>MKRRVVITGVGVRAPGGNGTRQFWELLTSGRTATRRISFFDPSPYRSQVAAEADFDPVAEGFGPRELDRMDRASQFAVACAREAFAASGLDPDTLDPARVGVSLGSAVAAATSLEREYLLLSDSGRDWEVDAAWLSRHMFDYLVPSVMPAEVAWAVGAEGPVTMVSTGCTSGLDSVGNAVRAIEEGSADVMFAGAADTPITPIVVACFDAIRATTARNDDPEHASRPFDGTRDGFVLAEGAAMFVLEDYDSALARGARIHAEISGYATRCNAYHMTGLKADGREMAETIRVALDESRTDATDIDYINAHGSGTRQNDRHETAAYKRALGEHARRTPVSSIKSMVGHSLGAIGSLEIAACVLALEHGVVPPTANLRTSDPECDLDYVPLEARERKLRSVLTVGSGFGGFQSAMVLRDAETAGAAA[4x];>[4x]MDYKDDDDKSVLITGVGVVAPNGLGLAPYWSAVLDGRHGLGPVTRFDVSRYPATLAGQIDDFHAPDHIPGRLLPQTDPSTRLALTAADWALQDAKADPESLTDYDMGVVTANACGGFDFTHREFRKLWSEGPKSVSVYESFAWFYAVNTGQISIRHGMRGPSSALVAEQAGGLDALGHARRTIRRGTPLVVSGGVDSALDPWGWVSQIASGRISTATDPDRAYLPFDE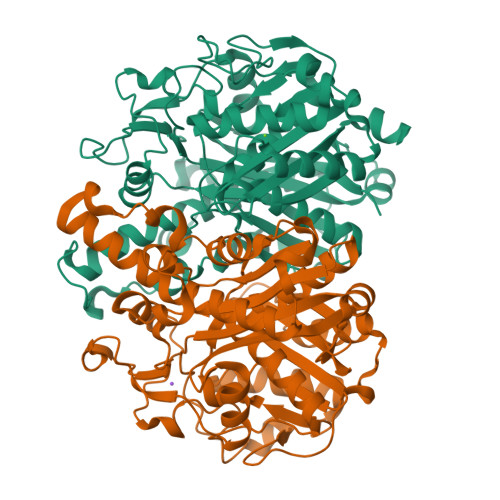RAAGYVPGEGGAILVLEDSAAAEARGRHDAYGELAGCASTFDPAPGSGRPAGLERAIRLALNDAGTGPEDVDVVFADGAGVPELDAAEARAIGRVFGREGVPVTVPKTTTGRLYSGGGPLDVVTALMSLREGVIAPTAGVTSVPREYGIDLVLGEPRSTAPRTALVLARGRWGFNSAAVLRRFAPTP>MRIIMPVEFSRIVRDVERLIAVEKYSLQGVVDGDKLLVVGFSEGSVNAYLYDGGETVKLNREPINSVLDPHYGVGRVILVRDVSKGAEQHALFKVNTSRPGEEQRLEAVKPMRILSGVDTGEAVVFTGATEDRVALYALDGGGLRELARLPGFGFVSDIRGDLIAGLGFFGGGRVSLFTSNLSSGGLRVFDSGE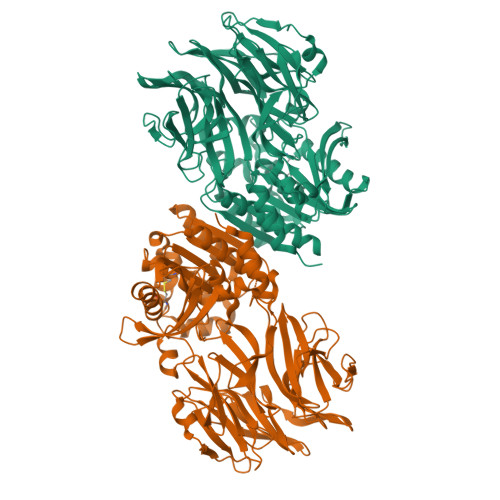GSFSSASISPGMKVTAGLETAREARLVTVDPRDGSVEDLELPSKDFSSYRPTAITWLGYLPDGRLAVVARREGRSAVFIDGERVEAPQGNHGRVVLWRGKLVTSHTSLSTPPRIVSLPSGEPLLEGGLPEDLRRSIAGSRLVWVESFDGSRVPTYVLESGRAPTPGPTVVLVHGGPFAEDSDSWDTFAASLAAAGFHVVMPNYRGSTGYGEEWRLKIIGDPCGGELEDVSAAARWARESGLASELYIMGYSYGGYMTLCALTMKPGLFKAGVAGASVVDWEEMYELSDAAFRNFIEQLTGGSREIMRSRSPINHVDRIKEPLALIHPQNASRTPLKPLLRLMGELLARGKTFEAHIIPDAGHAINTMEDAVKILLPAVFFLATQRERR[4x]> GPRVV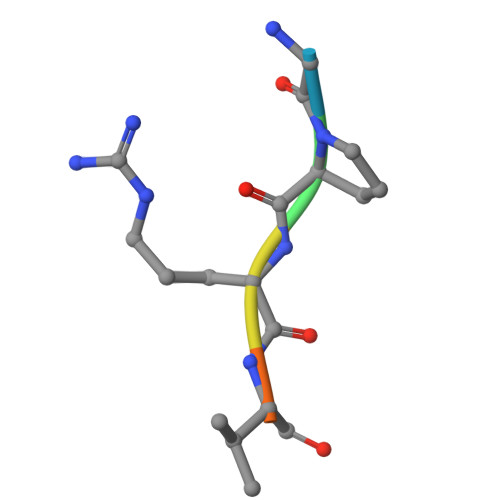E> AAPFNG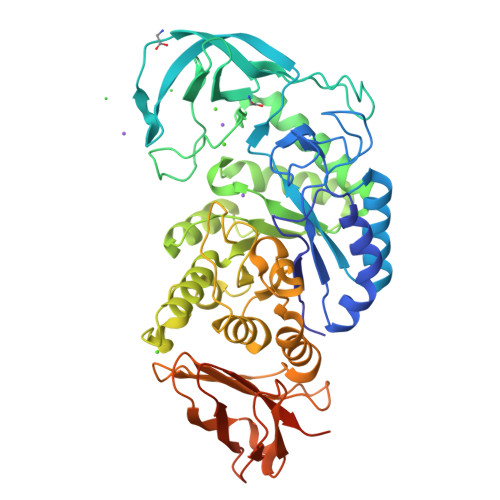TMMQYFEWYLPDDGTLWTKVANEANNLSSLGITALWLPPAYKGTSRSDVGYGVYDLYDLGEFNQKGTVRTKYGTKAQYLQAIQAAHAAGMQVYADVVFDHKGGADGTEWVDAVEVNPSDRNQEISGTYQIQAWTKFDFPGRGNTYSSFKWRWYHFDGVDWDESRKLSRIYKFRGKAWDWEVDTEFGNYDYLMYADLDMDHPEVVTELKNWGKWYVNTTNIDGFRLDAVKHIKFSFFPDWLSYVRSQTGKPLFTVGEYWSYDINKLHNYITKTDGTMSLFDAPLHNKFYTASKSGGAFDMRTLMTNTLMKDQPTLAVTFVDNHDTEPGQALQSWVDPWFKPLAYAFILTRQEGYPCVFYGDYYGIPQYNIPSLKSKIDPLLIARRDYAYGTQHDYLDHSDIIGWTREGGTEKPGSGLAALITDGPGGSKWMYVGKQHAGKVFYDLTGNRSDTVTINSDGWGEFKVNGGSVSVWVPRKTTVSTIARPITTRPWTGEFVRWTEPRLVAWP>MRKEAIHHRSTDNFAYAYDSETLHLRLQTKKNDVDHVELLFGDPYEWHDGAWQFQTMPMRKTGSDGLFDYWLAEVKPPYRRLRYGFVLRAGGEKLVYTEKGFYHEAPSDDTAYYFCFPFLHRVDLFQAPDWVKDTVWYQIFPERFANGNPAISPKGARPWGSEDPTPTSFFGGDLQGIIDHLDYLADLGITGIYLTPIFRAPSNHKYDTADYFEIDPHFGDKETLKTLVKRCHEKGIRVMLDAVFNHCGYEFAPFQDVLKNGAASRYKDWFHIREFPLQTEPRPNYDTFAFVPHMPKLNTAHPEVKRYLLDVATYWIREFDIDGWRLDVANEIDHQFWREFRQAVKALKPDVYILGLIWHDAMPWLRGDQFDAVMNYPLADAALRFFAKEDMSASEFADRLMHVLHSYPKQVNEAAFNLLGSHDTPRLLTVCGGDVRKVKLLFLFQLTFTGSPCIYYGDEIGMTGGNDPECRKCMVWDPEKQNKELYEHVKQLIALRKQYRALRRGDVAFLTADDEVNHLVYAKTDGNETVMIIINRSNEAAEIPMPIDARGKWLVNLLTGERFAAE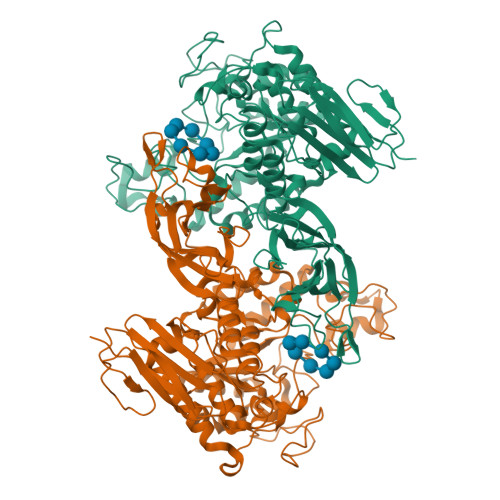AETLCVSLPPYGFVLYAVESW[2x]>APDWVPPEVFDLVAEDKARCMSEHGTTQAQIDDVAKGNLVNEPSITCYMYCLLEAFSLVDDEANVDEDIMLGLLP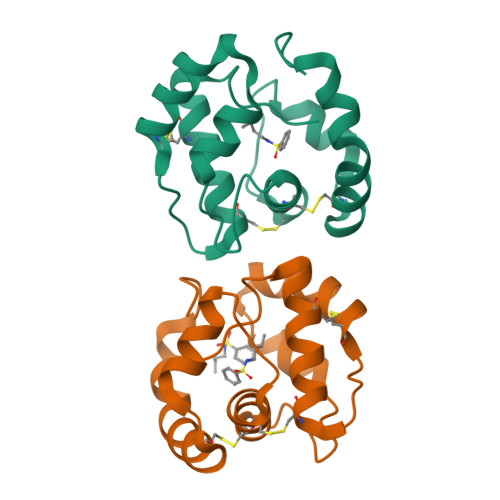DQLQERAQSVMGKCLPTSGSDNCNKIYNLAKCVQESAPDVWFVI[2x]> MILSAEQSFTLRHPHGQAAALAFVREPAAALAGVQRLRGLDSD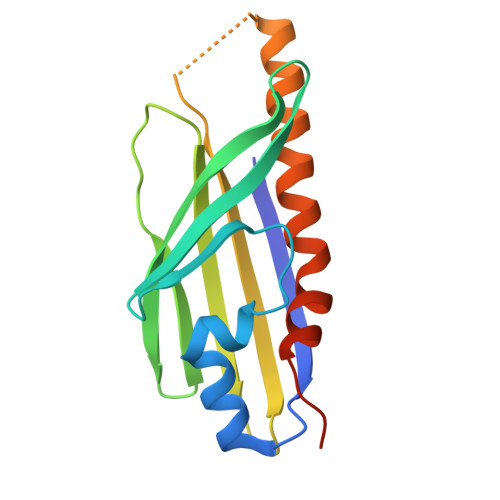GEQVWGELLVRVPLLGEVDLPFRSEIVRTPQGAELRPLTLTGERAWVAVSGQATAAEGGEMAFAFQFQAHLATPEAEGEGGAAFEVMVQAAAGVTLLLVAMALPQGLAAGLPPALEHHHHHH> MADAGKREGRVFAPYSVFKGAAALSAEPRLPTFNRLDSGGVKLNRRGVIMLTFWPSVGERKYDWEKRQLFALSATEVGSLISMGTRDSSEFFHDPSMLSSNAGQVRKSLSIKPNADGSGYF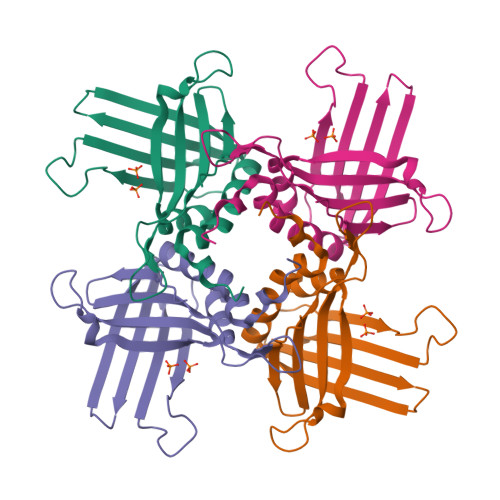ISLSVVNNNLKTNDRFTVPVTTAEFAVMRTAFSFALPHIMGWDRFTNRPLEHHHHHH>HHHHHHFNLPPGNYK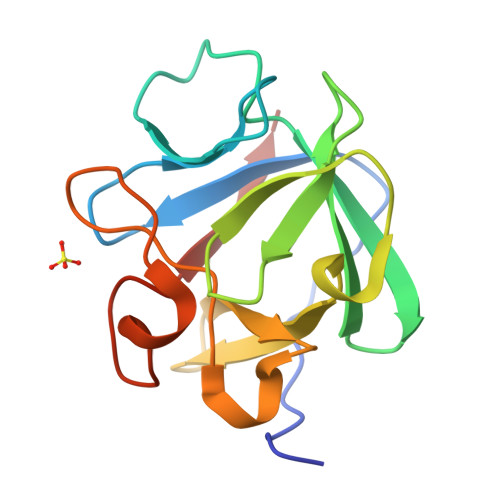KPKLLYCSNGGHFLRINPAGTVDGTRDRSDQHIQLQLSAESVGEVYIKSTETGQYLAMDTDGLLYGSQTPNEECLFLERLEENHYNTYISKKHAEKNWFVGLKKNGSCKRGPRTHYGQKAILFLPLPVSSD[2x]(1S)-1-(7-amino-1H-pyrazolo[4,3-d]pyrimidin-3-yl)-1,4-anhydro-D-ribitol | C10 H13 N5 O4 | 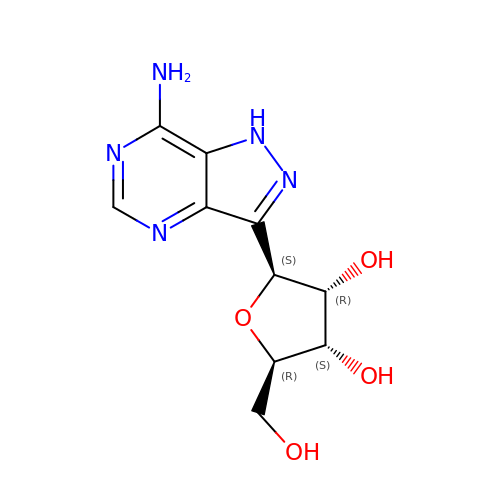KBHMEHLJSZMEMI-KSYZLYKTSA-N~{N}-[3-[[5-ethanoyl-2-[2-(2-oxa-6-azaspiro[3.3]heptan-6-yl)ethoxy]phenyl]carbamoyl]-5-(1-methylpyrazol-3-yl)phenyl]furan-2-carboxamide 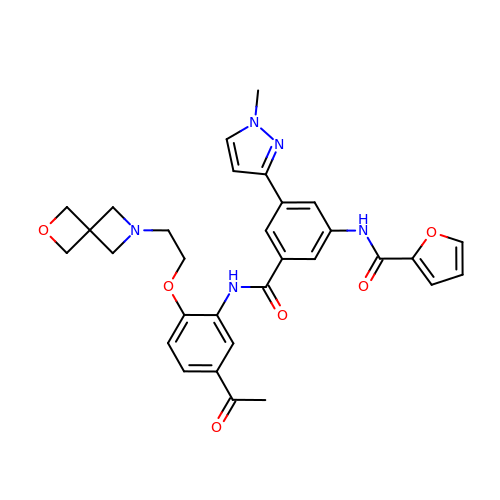| C31 H31 N5 O6 | VJMNNCAJWFIBNF-UHFFFAOYSA-N>[7x]MSDK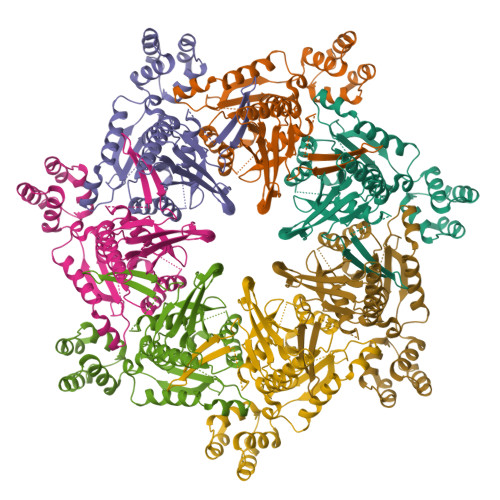PIDIQYDKQATPNLSGVITPPTNETGNDSVREKLSKLVGDAMSNNPYFAAGGGLMILGTGLAVARSGIIKASRVLYRQMIVDLEIQSKDKSYAWFLTWMAKHPQRVSRHLSVRTNYIQHDNGSVSTKFSLVPGPGNHWIRYKGAFILIKRERSAKMIDIANGSPFETVTLTTLYRDKHLFDDILNEAKDIALKTTEGKTVIYTSFGPEWRKFGQPKAKRMLPSVILDSGIKEGILDDVYDFMKNGKWYSDRGIPYRRGYLLYGPPGSGKTSFIQALAGELDYNICILNLSENNLTDDRLNHLMNNMPERSILLLEDIDAAFNKRSQTGEQGFHSSVTFSGLLNALDGVTSSEETITFMTTNHPEKLDAAIMRPGRIDYKVFVGNATPYQVEKMFMKFYPGETDICKKFVNSVKELDITVSTAQLQGLFVMNKDAPHDALKMVSSLRNANHIF> AACGGGCGCAGAA;>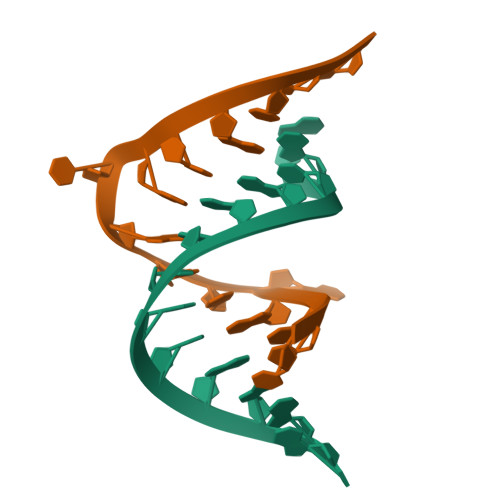 UCUGACGGUACGUUU> MKYQASKNRYNEMKYSKCGESGLKLPMISFGLWHNFGSNADYNNMKELCF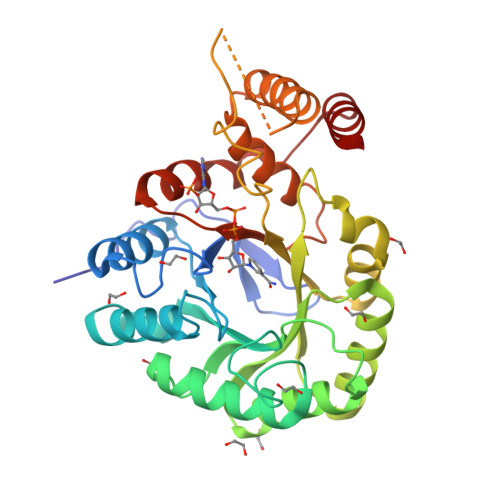TAFDNGITHFDLANNYGPVPGSAEENFGRILRDDLATYRDELLISTKAGYKMWEGPYGDFGSRKYILASLDQSLKRMGLEYVDIFYHHRMDPDTPLEESMMALDTAVKSGKALYAGISNYNGETMEKAAAILNELKCPFVINQNRYSIFDRTIENNGLKRAAKENGKGIIAFSPLAQGTLTDKYLSGIPDDSRIKVDGRFLKQDILTEKKLEQIRRLNNIALNRGQTLAQMALSWVLKDSEVTSVLIGASKPSQIIENVGIVHKIGFTDEELMMIDEISAN> GVALGATRVIYPAGQKQEQLAVTNNDENSTYLIQSWVENADGVKDGRFIVTPPLFAMKGKKENTLRILDATNNQLPQDRESLFWMNVKAIPSMDKSKLTENTLQLAIISRIKLYYRPAKLALPPDQAAEKLRFRRSANSLTLINPTPYYLTVTELNAGTRVLENALVPP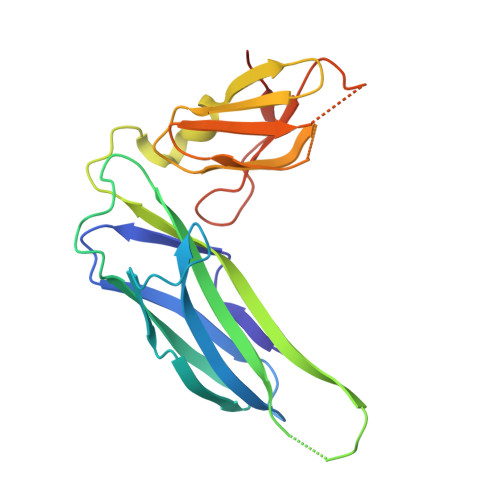MGESTVKLPSDAGSNITYRTINDYGALTPKMTGVMEHHHHHH> 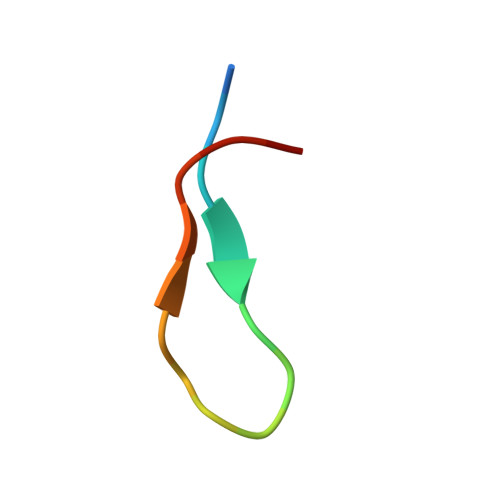XWRPRVARWTGQIIYCSX>[2x]SRVDGGMSVTLHTDVGDIKIEVFCERTPKTCENFLALCASNYYNGCIFHRNIKGFMVQTGDPTGTGRGGNSIWGKKFEDEYSEYLKHNVRGVVSMANNGPNTN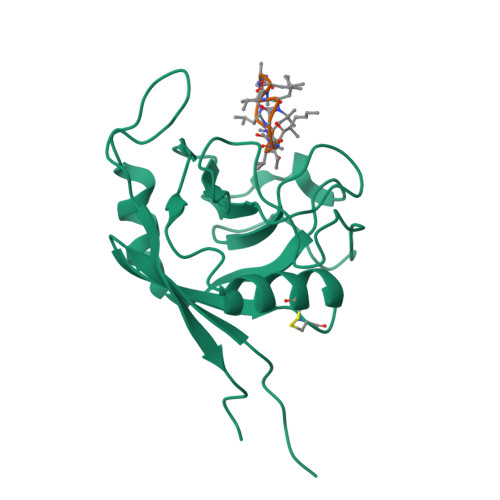GSQFFITYGKQPHLDMKYTVFGKVIDGLETLDELEKLPVNEKTYRPLNDVHIKDITIHANPFAQ;>[2x]ALLVTAGLVLA> MVVRSWRHMKERYNLIGTRCKTCGKVYFPSRTVCPDCRRKGELEEFQLSGKGKIY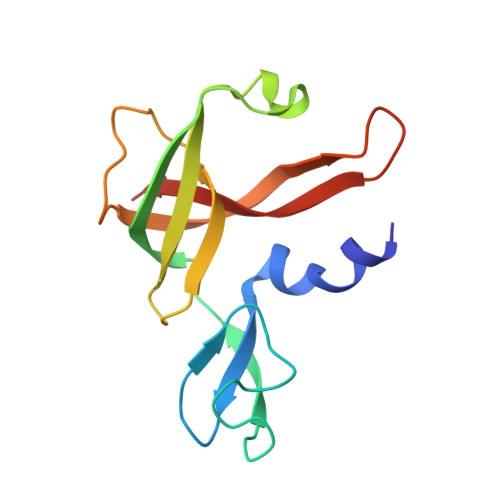TYSIVYAPPKEFNKLTPYVIAIVELEEGPKVTAQVDCDINKISIGIPVEAAFRRIKEDGKDGIISYGYKFVPITE Meprins (Meprin α and β) are multidomain, Zn-dependent proteases. They belong to the astacin family and metzincin superfamily of endo-proteinases. Originally discovered in the early 1980s in human intestine and mouse kidney, Meprins have only been described in vertebrate tissue such as human skin, leukocytes and various cancer cells. They are involved in a broad range of proteolytic processes, among these connective tissue homeostasis and immunological and intestinal barrier function. Meprin β shows a striking preference for negatively charged amino acids proximal to the scissile bond.

To investigate this interaction in detail, we crystallized the catalytically active ectodomain of human Meprin β in complex with the tertiary-amine inhibitor MWT-S-270. The mature Meprin β variant Meprin β62–595 (MβΔC) crystallized in the presence of MWT-S-270 in two different space groups, the already reported hexagonal space group P6122 (178) (data not shown) and, additionally, under the conditions reported here, in the monoclinic space group C2 (5), with two monomers in the asymmetric unit. Each monomer spans the catalytic active protease domain (Asn62-Leu259), the MAM-domain (Ser260-Cys427) and the TRAF-domain (Pro428-Gln595). Both monomers are covalently linked through an intermolecular disulfide bridge connecting residue Cys305 of monomer A and B. This feature could not be observed in the crystal structure described previously. Each monomer comprises at least three bound metal ions: two tentative calcium ions and a catalytic zinc ion. The hydroxamic acid moiety is bound to the zinc ion in a bidentate fashion, which is commonly observed with these inhibitors. One benzyl residue is directed to the S1-site, while the second benzyl residue of the tertiary amine is directed towards the S1′-subsite, shaped by Arg238. The unexpected interaction is a fixation of the benzoic acid moiety within the S1′-site via a network of hydrogen bonds, i.e., the sidechain OH of Ser212 at a distance of 2.8–2.9 Å, the backbone NH of Ser212 at a distance of 3.2 Å and a water-bridged hydrogen bond with Thr214 at a distance of 2.6 and 2.8 Å. The closest distance between the carboxylic acid and the guanidinium moiety of Arg184 is around 4 Å, albeit the electron density for the C11, C12 and C13 of MWT-S-270 in monomer A and C8, C9 and C13 in monomer B is not defined, and the moiety of the inhibitor is probably highly flexible via rotation around the single bond connecting C7-C8. Moreover, the whole loop forming the lower rim of the active site cleft, harboring Arg184, is also less well resolved, as reflected by higher B-factors, especially in monomer B. The missing electron density of the side chain of Arg184 in monomer B and the barely resolved Arg184 in monomer A (together with the less well resolved whole loop) led us to conclude a high degree of flexibility.

>NSIIGEKYRWPHTIPYVLEDSLEMNAKGVILNAFERYRLKTCIDFKPWAGETNYISVFKGSGCWSSVGNRRVGKQELSIGANCDRIATVQHEFLHALGFWHEQSRSDRDDYVRIMWDRILSGREHNFNTYSDDISDSLNVPYDYTSVMHYSKTAFQNGTEPTIVTRISDFEDVIGQRMDFSDSDLLKLNQLYNCSSSLSFMDSCSFELENVCGMIQSSGDNADWQRVSQVPRGPESDHSNMGQCQGSGFFMHFDSSSVNVGATAVLESRTLYPKRGFQCLQFYLYNSGSESDQLNIYIREYSADNVDGNLTLVEEIKEIPTGSWQLYHVTLKVTKKFRVVFEGRKGSGASLGGLSIDDINLSETRCPHHIWHIRNFTQFIGSPNGTLYSPPFYSSKGYAFQIYLNLAHVTNAGIYFHLISGANDDQLQWPCPWQQATMTLLDQNPDIRQRMSNQRSITTDPFMTTDNGNYFWDRPSKVGTVALFSNGTQFRRGGGYGTSAFITHERLKSRDFIKGDDVYILLTVEDISHLNSTQ[2x]N'-[(1E)-(3,5-dibromo-2,4-dihydroxyphenyl)methylidene]naphthalene-2-carbohydrazide | C18 H12 Br2 N2 O3 | 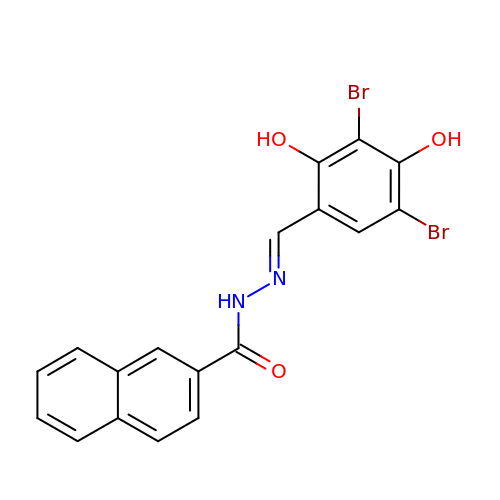LVLHTGJPIBVDTM-ZVBGSRNCSA-N>MTLKQVIV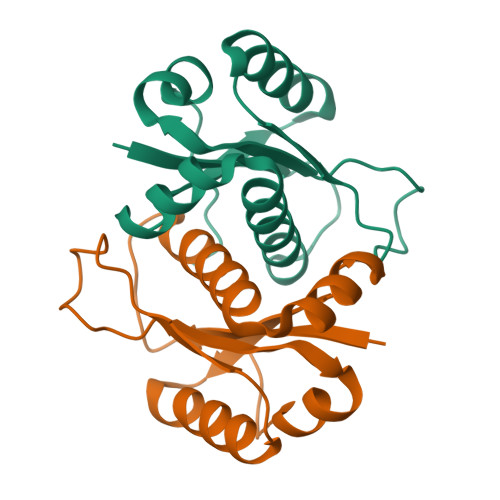VRDDLKLSRGKLAVQVAHAAIIGYLKSDSSLRRKWLDEGQKKVVLKVKSLEELLGIKHKAESLGLVTGLVQDAGLTEVPPGTITAVVIGPDEERKIDKVTGNLPLLKLEHHHHHH[2x]>[4x]APNYKLTYFNMRGRAEIIRYIFAYLDIQYEDHRIEQADWPEIKSTLPFGKIPILEV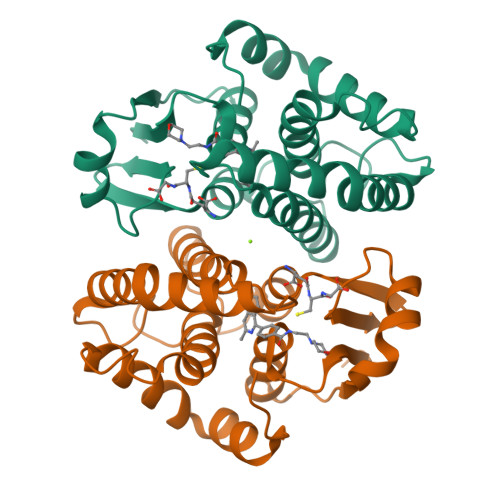DGLTLHQSLAIARYLTKNTDLAGNTEMEQCHVDAIVDTLDDFMSCFPWAEKKQDVKEQMFNELLTYNAPHLMQDLDTYLGGREWLIGNSVTWADFYWEICSTTLLVFKPDLLDNHPRLVTLRKKVQAIPAVANWIKRRPQTKL> SLMRVQ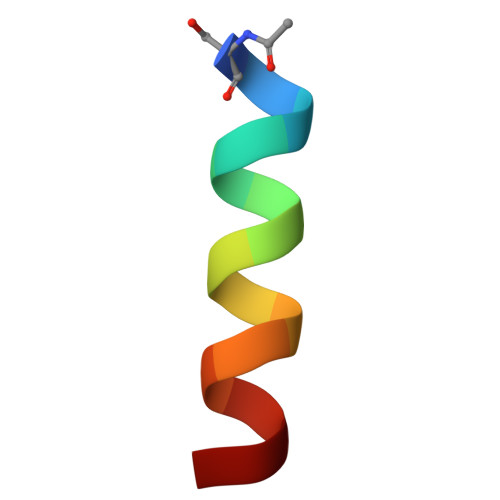AHIRKRMVA6-methylpyrazolo[1,5-a]pyrimidine-3-carboxamide | C8 H8 N4 O | 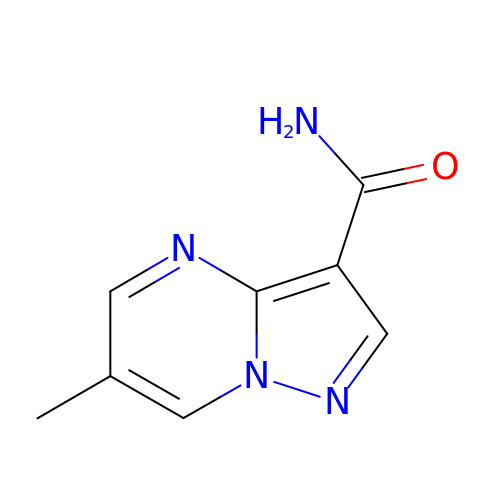ZSJDYGZWDYMLDS-UHFFFAOYSA-N> MNDLMLDKSALLFGVSKYLEKGIITGNVLIHKSLL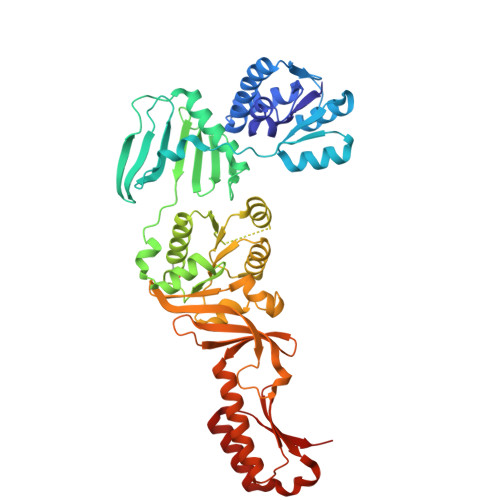AELERESNDGLVSAEIALDEVKKLKDITERILVNFEIVGDDSKKGEANELSREYCLEKGCIIVTADETQKKICDAMGIQYNFLQPLKQGLSFESFFDDETMSLHIKEDTVPKAKKGKPGNWKFVNLSDKPMLSTDVRMIANEIINAVRLIKGSFVEIERRGSLSIQLGNYAVVITRPPLSDGWEITITRPVVRKRLEDYNLDERLIKRLEERAEGIIIAGAPGMGKTTFAQALAEYYMRLGKIVKTIESPRDMHLPPEITQYSKNYAEIGELHDILLLSRPDYTVYDEMRNDEDFKLYVDLRLAGVGMVGVVHATSPIDAIHRFVNRVDIGTIPNILDTIIFINSGNVSKVYTLEMTVKVPAGLKEADLARPVVEIKDLATGNTEYEIYVFGEQTMIVPVNRGITMSNMEFKISKIVNNIIPNATVKYEDGEYVIVIPKEEIGKYNRKLVQRLKRLEKKNNIKIKIKLSD>GAGEARLEEAVNRWVLKFYFHEALRAFRGSRYGDFRQIRDIMQALLVRPLGKEHTVSRLLRVMQCLSRIEEGENLDCSFDMEAELTPLESAINVLEMIKTEFTLTEAVVESSRKLVKEAAVIICIKNKEFEKASKILKKHMSKDPTTQKLRNDLLNIIREKNLAHPVIQNFSYETFQQKMLRFLESHLDDAEP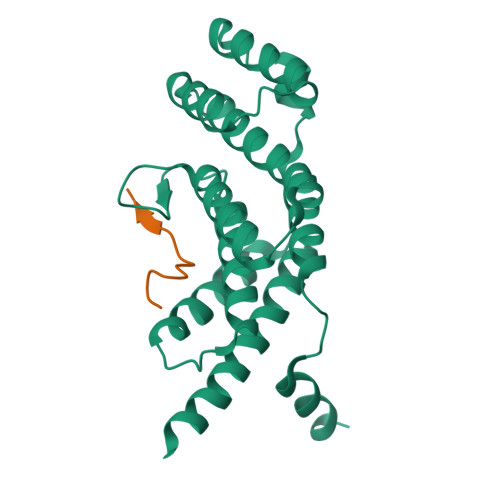YLLTMAKKALK[7x];>KMRIPNYQLSPTKLPS[7x]>ASLTEIEHLVQSVCKSYRETCQLRLEDLLRQRSNIFSREEVTGYQRKSMWEMWERCAHHLTEAIQYVVEFAKRLSGFMELCQNDQIVLLKAGAMEVVLVRMCRAYNADNRTVFFEGKYGGMELFRALGCSELISSIFDF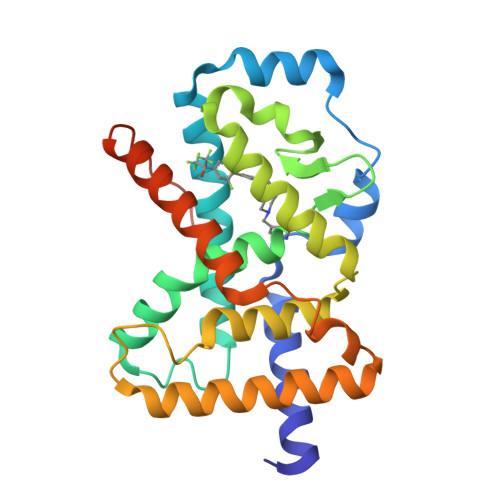SHSLSALHFSEDEIALYTALVLINAHRPGLQEKRKVEQLQYNLELAFHHHLCKTHRQSILAKLPPKGKLRSLCSQHVERLQIFQHLHPIVVQAAFPPLYKELFSGN[2x]>[4x]GMSTSPA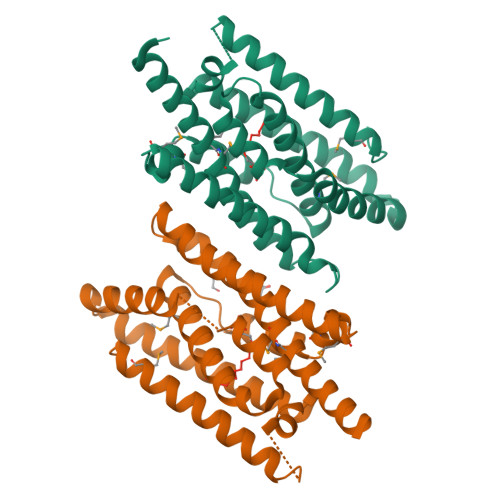DTARYNRFVADLFGMMAYGELSAFERFSADARYSPTLHDRAVLGRIAVVEFRHYELVSARLEAMGIDAEDAMLPFQAAVDYFHSRTRPADWYESLMKAYVIDTVSADFYRAISRYVDAGTRDVIEQIQASDETTEVLRERLRSALADDPRLASRLALWGRRLLGEALTQAQRVSYEHAFLGSLIGGEDSAAAKELVSGLIAGLAEKHSKRMTQLGLTG>[4x]HHHHHHGSQIHVDTMKVINDPIHGHIELHPLLVRIIDTPQFQRLRYIKQLGGGYYVFPGASHNRFEHSLGVGYLAGCLVHALGEKQPELQISERDVLCVQIAGLCHDLGHGPFSHMFDGRFIPLARPEVKWTHEQGSVMMFEHLINSNGIKPVMEQYGLIPEEDIYFIKEQIVGPLESPVEDSLWPYKGRPENKSFLYEIVSNKRNGIDVDKWDYFARDCHHLGIQNNFDYKRFIKFARVCEVDNELRICARDKEVGNLYDMFHTRNSLHRRAYQHKVGNIIDTMITDAFLKADDYIEITGAGGKKYRISTAIDDMEAYTKLTDNIFLEILYSTDPKLKDAREILKQIEYRNLFKYVGETQPTGQIKIKREDYESLPKEVASAKPKVLLDVKLKAEDFIVDVINMD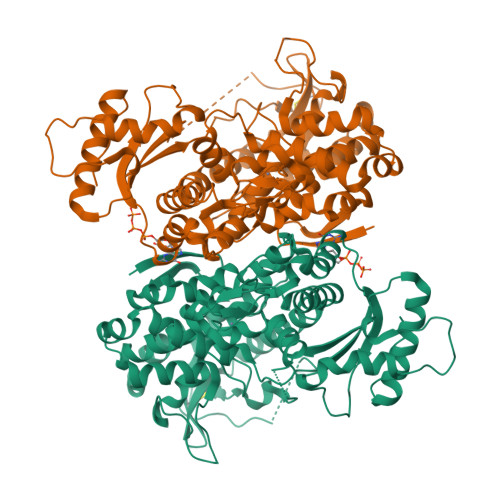YGMQEKNPIDHVSFYCKTAPNRAIRITKNQVSQLLPEKFAEQLIRVYCKKVDRKSLYAARQYFVQWCADRNFTKPQDGDVIAPLITPQKKEWNDSTSVQNPTRLREASKSRVQLFKDDPM> EDLCRAPD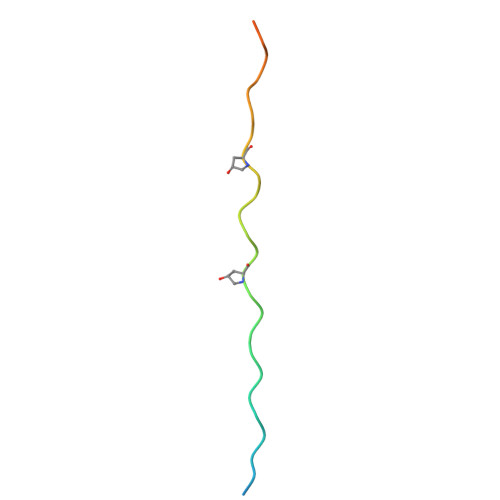GKKGEAGRPGRRGRPGLKGQGEPGAPGIR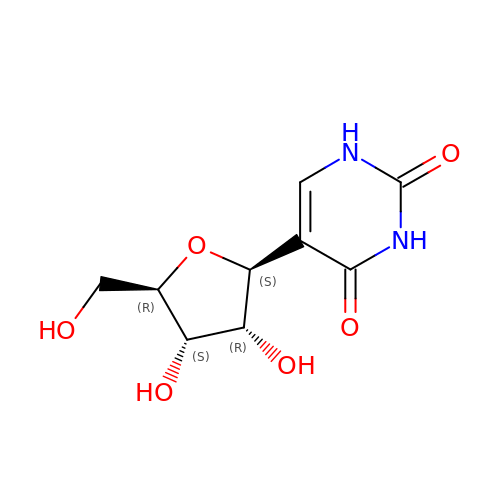5-[(2~{S},3~{R},4~{S},5~{R})-5-(hydroxymethyl)-3,4-bis(oxidanyl)oxolan-2-yl]-1~{H}-pyrimidine-2,4-dione | C9 H12 N2 O6 | PTJWIQPHWPFNBW-GBNDHIKLSA-N> MLKELLRSLKASMGIYEARDGSIYGLLAEFSDPAALLHAARQVRKA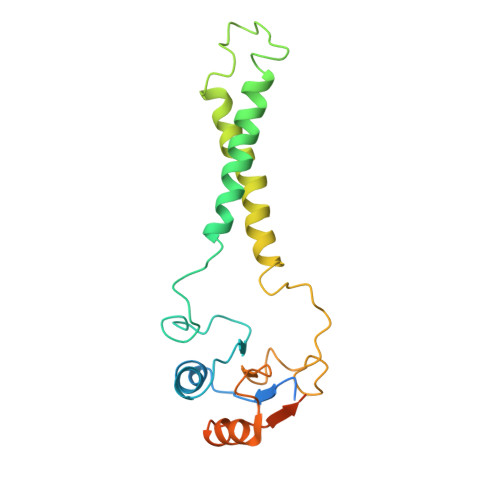GYRHFDAHSPFPIHGMDEAMGLGNSKVAFITFFTGTIAGFALAWWMQWWMGAVDYPLNISGKPFFALPPSVPIIFELTILFSALAGVATMLALNGLPRPYNPLFYSKNFMRVTDDGFFLFVAASDPKFDPTATRQLLEQLGGYNIEVIEDRGEEDVTPATAPAAEAAVTTS> MGSSHHHHHHSQDPNSSSARLQVDKLDYDIPTTENLYFQGSMRRSVYLDNTIEFLRGRVYLGAYDYTPEDTDELVFFTVEDAIFYNSFHLDFGPMNIGHLYRFAVIFHEILNDPENANKAVVFYSSASTRQRANAACMLCCYMILVQAWTPHQVLQPLAQVDPPFMPFRDAGYSNADFEITIQDVVYGVWRAKEKGLIDLHSFNLESYEKYEHVEFGDFNVLTPDFIAFASPQEDHPKGYLATKSSHLNQPFKSVLNFFANNNVQLVVR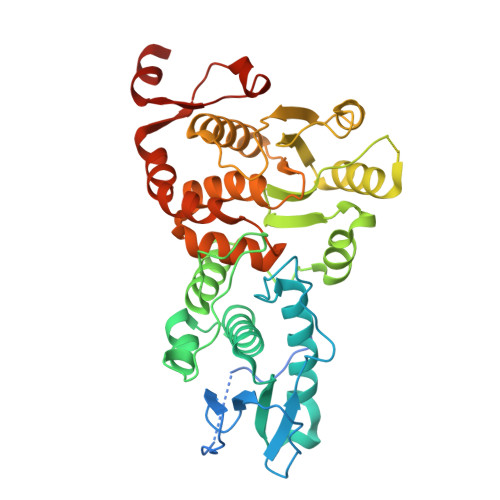LNSHLYNKKHFEDIGIQHLDLIFEDGTCPDLSIVKNFVGAAETIIKRGGKIAVHSKAGLGRTGCLIGAHLIYTYGFTANECIGFLRFIRPGMVVGPQQHWLYLHQNDFREWKYTTRISLKPSEAIGGLYPLISLEEYRLQKKKLKD>SNAMAKITVGTENQAPIEIYYEDHGTGKPVVLIHGWPLSGRSWEYQVPALVEAGYRVITYDRRGFGK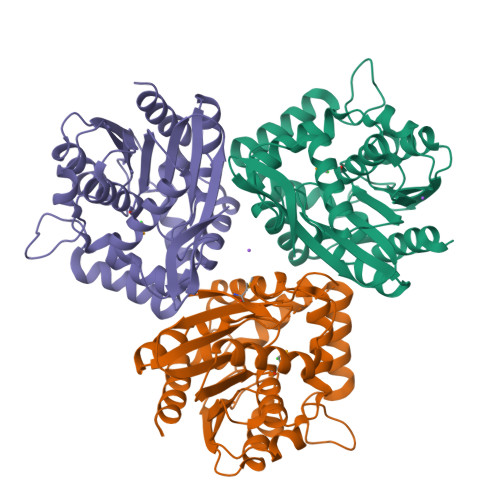SSQPWEGYEYDTFTSDLHQLLEQLELQNVTLVGFSMGGGEVARYISTYGTDRIEKVVFAGAVPPYLYKSEDHPEGALDDATIETFKSGVINDRLAFLDEFTKGFFAAGDRTDLVSESFRLYNWDIAAGASPKGTLDCITAFSKTDFRKDLEKFNIPTLIIHGDSDATVPFEYSGKLTHEAIPNSKVALIKGGPHGLNATHAKEFNEALLLFLKD[3x]> MAAGSRFPFCTAARLSSRGTLPRLGEATFFAGAESQRSA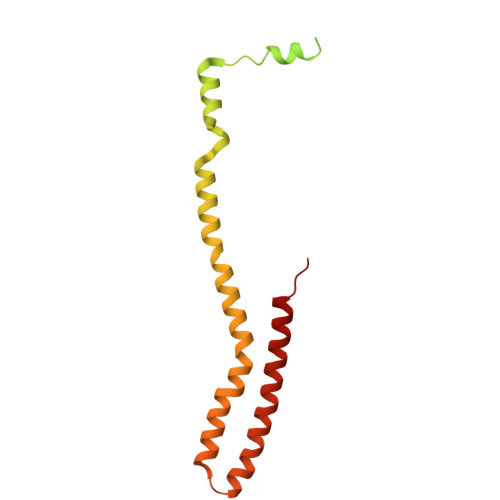GAFAKTLQRPFLRAPSTQLFPVGNRLGVSSARALVANAMEPRRFFAAAASAKATHALQPTGTGSVAFTRPGQGSNAQFQTSLADKTRGLLGVGFLRPTKMASFAATFLLNFRFYFMYMARTTFQAVRPLLAFSVFGEVMKLVLATMSSGLFSFLFSFVLAFEVFYFFLQCYISYTFLTMFFTVLF> SLKGMISVGPWGGSGGDHWSFKANHAITEILIHVKDNIKSISFKDAGGDISGTFGGKDPRENKKGEEKKIGIRWPTEYLKSISGSYGDYNGILVIRSLSFITNLTTYGPFGSTSGGESFSIPIADSVVVGFHGRAGYYLDALGIFVQPVPHRTISFGPWGGPAGDDAFNFKVGSWIKDIIVYADATINSIAFKDADGHCEKFGGQDPNDIGVEEKVEIDGNLEHLTSISGTYGNYKGFEVLTSLSFITNVTKHGPFGIASGTSFSRPIEGSLVTGFHGKGGYYLDSIGIYVKPRDVEGSISIGPWGGSGGDPWSYTANEGINQIIIYAGSNIKSIAFKDTSGLDSATFGGVNPKDTGEKNTVSIKWPSEYLTSIDGTYGQYKFKDVFTTVTSLSFTTNLATYGPFGKASLTSFSIPIHNNMVVGFHG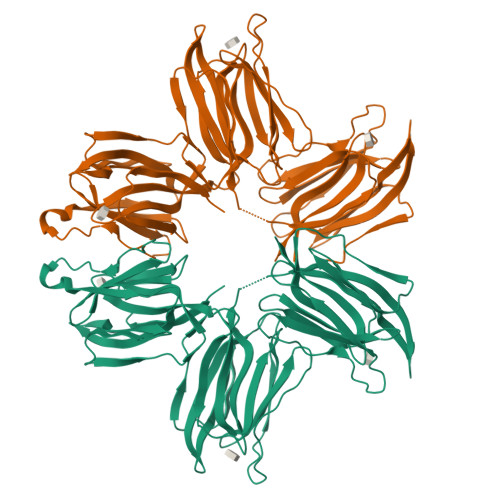RAGDYLDAIGIFVKPDTAV>MQLFDLPLDQLQTYKPEKTAPKDFSEFWKLSLEELAKVQAEPDLQPVDYPADGVKVYRLTYKSFGNARITGWYAVPD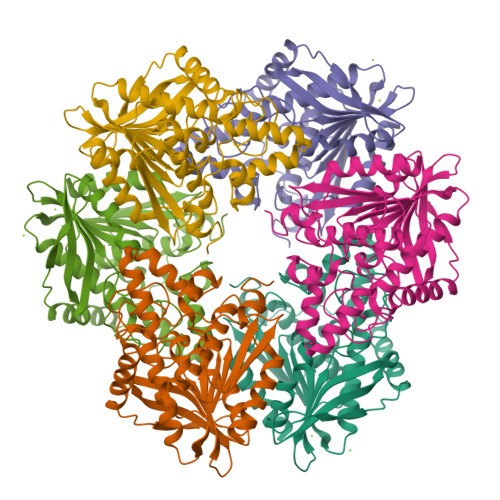KEGPHPAIVKYHGYNASYDGEIHEMVNWALHGYATFGMLVRGQQSSEDTSISPHGHALGWMTKGILDKDTYYYRGVYLDAVRALEVISSFDEVDETRIGVTGGSQGGGLTIAAAALSDIPKAAVADYPYLSNFERAIDVALEEPYLEINSFFRRNGSPETEVQAMKTLSYFDIMNLAYRVKVPVLMSIGLIDKVTPPSTVFAAYNHLETKKELKVYRYFGHEYIPAFQTEKLAFFKQHLKG[8x]> MNPNNRSEHDTIKTTENNEVPTNHVQYPLAETPNPTLEDLNYKEFLRMTADNNTEALDSSTTKDVIQKGISVVGDLLGVVGFPFGGALVSFYTNFLNTIWPSEDPWKAFMEQVEALMDQKIADYAKNKALAELQGLQNNVEDYVSALSSWQKNPVSSRNPHSQGRIRELFSQAESHFRNSMPSFAISGYEVLFLTTYAQAANTHLFLLKDAQIYGEEWGYEKEDIAEFYKRQLKLTQEYTDHCVKWYNVGLDKLRGSSYESWVNFNRYRREMTLTVLDLIALFPLYDVRLYPKEVKTELTRDVLTDPIVGVNNLRGYGTTFSNIENYIRKPHLFDYLHRIQFHTRFQPGYYGNDSFNYWSGNYVSTRPSIGSNDIITSPFYGNKSSEPVQKLEFKGEKVYRAVANTNLAVWPSAVYSGVTKVKFSQYNDKTKKASKQTYDSKRNVGAVSWDSIDQLPPETKKKPLKKGYSHQLNYVMCFLMQGSRGTIPVLTWTHKSVDFFNMIDSKKITQLPLVKAYKLQSGASVVAGPRFTGGDIIQCTENGSAATIYVTPDVSYSQKYRARIHYASTSQITFTLSLDGAPFNQYYFDKTINKGDTLTYNSFNLASFSTPFELS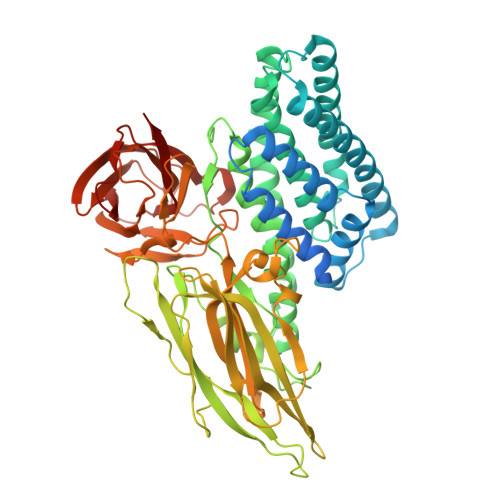GNNLQIGVTGLSAGDKVYIDKIEFIPVN> SLPREDTVYIGGALWGPATTWNLYAPQSTWGTDQFMYLPAFQYDLGRDAWIPVIAERYEFVDDKTLRIYIRPEARWSDGVPITADDFVYALELTKELGIGPGGGWDTYIEYVKAVDTKVVEFKAKEENLNYFQFLSYSLGAQPMPKHVYERIRAQMNIKDWINDKPEEQVVSGPYKLYYYDPNIVVYQRVDDWWGKDIFGLPRPKYLAHVIYKDNPSASLAFERGDIDWNGLFIPSVWELWEKKGLPVGTWYKKEPYFIPDGVGFVYVNNTKPGLSDPAVRKAIAYAIPYNEMLKKAYFGYGSQAHPSMVIDLFEPYKQYIDYELAKKTFGTEDGRIPFDLDMANKILDEAGYKKGPDGVRVGPDGTKLGPYTISVPYGWTDWMMMCEMIAKNLRSIGIDVKTEFPDFSVWADRMTKGTFDLIISWSVGPSFDHPFNIYRFVLDKRLSKPVGEVTWAGDWERYDNDEVVELLDKAVSTLDPEVRKQAYFRIQQIIY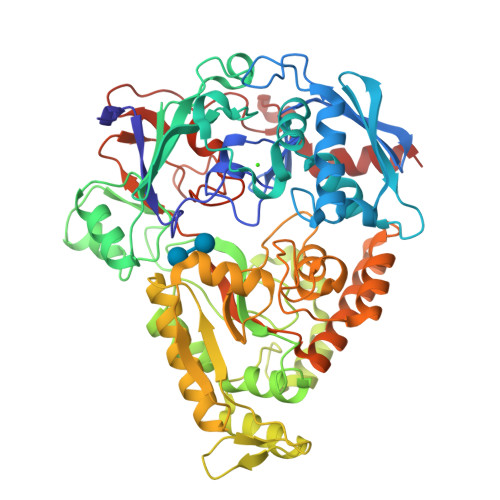RDMPSIPAFYTAHWYEYSTKYWINWPSEDNPAWFRPSPWHADAWPTLFIISKKSDPQPVPSWLGTVDEGGIEIPTAKIFEDLQKAT> XKGFVCPPEW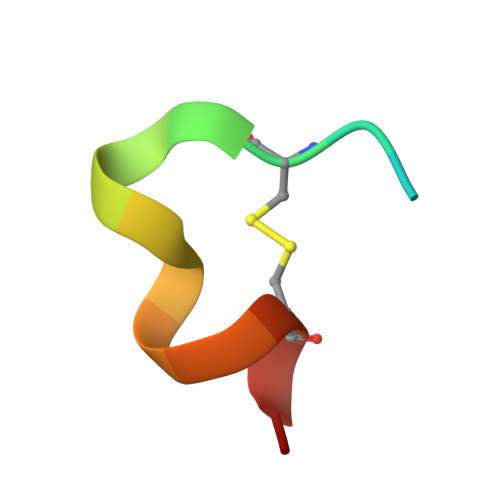RWLCDLX>[3x]MYSKIKISGTIEVVTGLHIGGGGESSMIGAIDSPVVRDLQTKLPIIPGSSIKGKMRNLLAKHFGLKMKQESHNQDDERVLRLFGSSEKGNIQRARLQISDAFFSEKTKEHFAQNDIAYTETKFENTINRLTAVANPRQIERVTRGSEFDFVFIYNVDEESQVEDDFENIEKAIHLLENDYLGGGGTRGNGRIQFKDTNIETVVGEYDSTNLKIK;> MTIKNYEVVIKTLGPIHIGSGQVMKKQ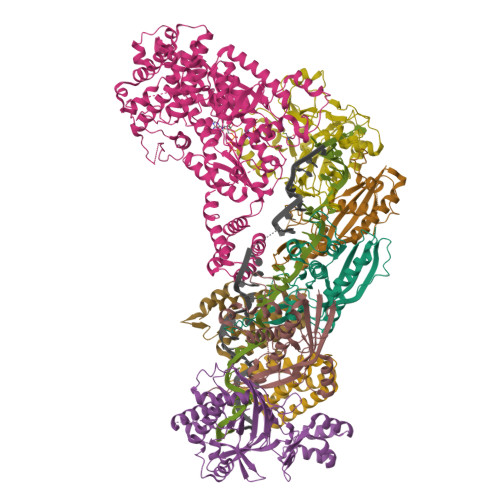DYIYDFYNSKVYMINGNKLVKFLKRKNLLYTYQNFLRYPPKNPRENGLKDYLDAQNVKQSEWEAFVSYSEKVNQGKKYGNTRPKPLNDLHLMVRDGQNKVYLPGSSIKGAIKTTLVSKYNNEKNKDIYSKIKVSDSKPIDESNLAIYQKIDINKSEKSMPLYRECIDVNTEIKFKLTIEDEIYSINEIEQSIQDFYKNYYDKWLVGFKETKGGRRFALEGGIPDVLNQNILFLGAGTGFVSKTTHYQLKNRKQAKQDSFEILTKKFRGTYGKMKEIPSNVPVALKGTTNQSRHTSYQQGMCKVSFQELNNEVL;> MNKKNILMYGSLLHDIGKIIYRSGDHTFSRGTHSKLGHQFLSQFSEFKDNEVLDNVAYHHYKELAKANLDNDNTAYITYIADNIASGIDRRDIIEEGDEEYEKQLFNFDKYTPLYSVFNIVNSEKLKQTNGKFKFSNESNIEYPKTENIQYSSGNYTTLMKDMSHDLEHKLSIKEGTFPSLLQWTESLWQYVPSSTNKNQLIDISLYDHSRITCAIASCIFDYLNENNIHNYKDELFSKYENTKSFYQKEAFLLLSMDMSGIQDFIYNISGSKALKSLRSRSFYLELMLEVIVDQLLERLELARANLLYTGGGHAYLLVSNTDKVKKKITQFNNELKKWFMSEFTTDLSLSMAFEKCSGDDLMNTSGNYRTIWRNVSSKLSDIKAHKYSAEDILKLNHFHSYGDRECKECLRSDIDINDDGLCSICEGIINISNDLRDKSFFVLSETGKLKMPFNKFISVIDYEEAEMLVQNNNQVRIYSKNKPYIGIGISTNLWMCDYDYASQNQDMREKGIGSYVDREEGVKRLGVVRADIDNLGATFISGIPEKYNSISRTATLSRQLSLFFKYELNHLLENYQITAIYSGGDDLFLIGAWDDIIEASIYINDKFKEFTLDKLTLSAGVGMFSGKYPVSKMAFETGRLEEAAKTGEKNQISLWLQEKVYNWDEFKKNILEEKLLVLQQGFSQTDEHGKAFIYKMLALLRNNEAINIARLAYLLARSKMNEDFTSKIFNWAQNDKDKNQLITALEYYIYQIREAD;> MTLATKVFKLSFKTPVHFGKKRLSDGEMTITADTLFSALFIETLQLGKDTDWLLNDLIISDTFPYENELYYLPKPLIKIDSKEEDNHKAFKKLKYVPVHHYNQYLNGELSAEDATDLNDIFNIGYFSLQTKVSLIAQETDSSADSEPYSVGTFTFEPEAGLYFIAKGSEETLDHLNNIMTALQYSGLGGKRNAGYGQFEYEIINNQQLSKLLNQNGKHSILLSTAMAKKEEIESALKEARYILTKRSGFVQSTNYSEMLVKKSDFYSFSSGSVFKNIFNGDIFNVGHNGKHPVYRYAKPLWLEV;>MTFAHEVVKSNVKNVKDRKGKEKQVLFNGLTTSKLRNLMEQVNRLYTIAFNSNEDQLNEEFIDELEYLKIKFYYEAGREKSVDEFLKKTLMFPIIDRVIKKESKKFFLDYCKYFEALVAYAKYYQKED[2x]> MTEAQAIAKQLGGVKPDDEWLQAEIARLKGKSIVPLQQVKTLHDWLDGKRKARKSCRVVGESRTGKTVACDAYRYRHKPQQEAGRPPTVPVVYIRPHQKCGPKDLFKKITEYLKYRVTKGTVSDFRDRTIEVLKGCGVEMLIIDEADRLKPETFADVRDIAEDLGIAVVLVGTDRLDAVIKRDEQVLERFRAHLRFGKLSGEDFKNTVEMWEQMVLKLPVSSNLK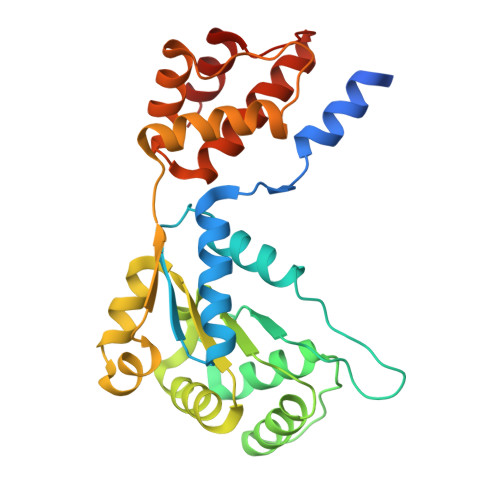SKEMLRILTSATEGYIGRLDEILREAAIRSLSRGLKKIDKAVLQEVAKEYK>[4x]MGSSHHHHHHSSENLYFQGHMSSRAETPRVPFLDLKAAYEELRAETDAAIARVLDSGRYLLGPELEGFEAEFAAYCETDHAVGVNSGMDALQLALRGLGIGPGDEVIVPSHTYIASWLAVSATGATPVPVEPHED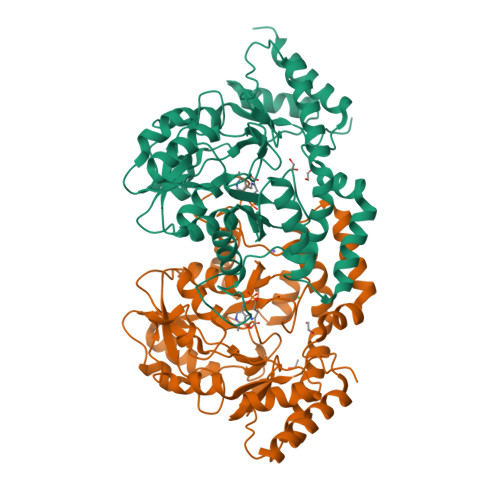HPTLDPLLVEKAITPRTRALLPVHLYGHPADMDALRELADRHGLHIVEDAAQAHGARYRGRRIGAGSSVAAFSFYPGKNLGCFGDGGAVVTGDPELAERLRMLRNYGSRQKYSHETKGTNSRLDEMQAAVLRIRLAHLDSWNGRRSALAAEYLSGLAGLPGIGLPVTAPDTDPVWHLFTVRTERRDELRSHLDARGIDTLTHYPVPVHLSPAYAGEAPPEGSLPRAESFARQVLSLPIGPHLERPQALRVIDAVREWAERVDQA>MYHCHSGSKPTEKGANEYAYAKWKLCSASAICFIFMIAEVVGGHIAGSLAVVTDAAHLLINLTSFLLSLFSLWLSSKPPSKRLTFGWHRAEILGALLSILCIWVVTGVLVYLACERLLYPDYQIQATVMIIVSSCAVAANIVLTVVLHQRCLGHNHKEVQANASVRAAFVHALGNLFQSISVLISALIIYFKPEYKIADPICTFIFSILVLASTITILKDFSILLMEGVPKSLNYSGVKELILAVDGVLSVHSLHIWSLTMNQVILSAHVATAASRDSQVVRREIAKALSKSFTMHSLTIQMESPVDQDPDCLFCEDPCD[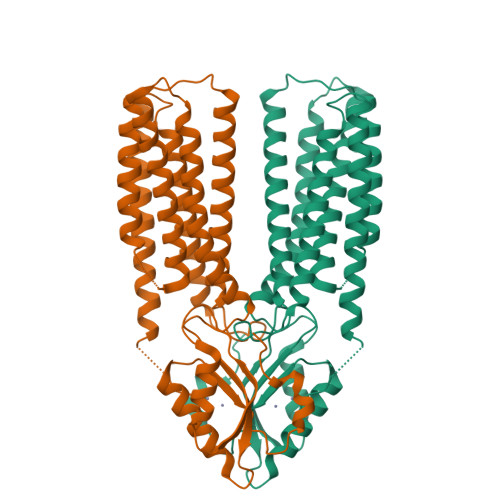2x]>MPMFTVNTNVPRASV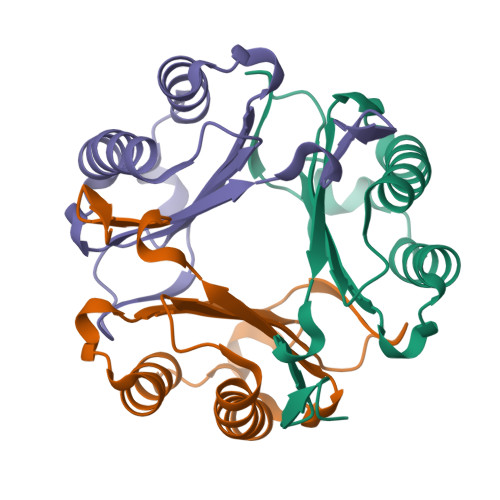PEGLLSELTQQLAQATGKPAQYIAVHVVPDQLMTFSGSSDPCALCSLHSIGKIGGAQNRTYSKLLCGLLADRLHISPDRIYINYYDMSAANVGWNGSTFALEHHHHHH[3x]> SASRDDWRAARSMHEFSAKDIDGHMVNLDKYRGFVSIVTNVASQCGKTEVNYTQLVDL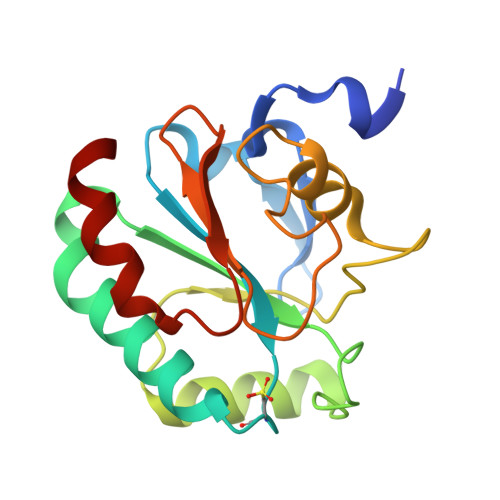HARYAERGLRILAFPSNQFGKQEPGSNEEIKEFAAGYNVKFDMFSKIEVNGDDAHPLWKWMKIQPKGKGILGNAIKWNFTKFLIDKNGVVVKRYGPMEEPLVIEKDLPHYF>[2x]MSVLPGAAAIAGIGATEFSKNSGRSELQLACEAVLAAIADAGLEPSDVDGLVTFTADTSSEIHVARNTGIGELKFFSRVGYGGGAACGTVQQAAMAVATGIAEVVVCYRAFNERSGVRYGLGQAGRQMDQGADSAAYAWLLPFGLNTPAQWVAMFARRYMHEYGATSEDFGRVAVVDRKHAATNPKAWFYQRPITLEDHQNSRWIVEPLHLLDCCQESDGGQALVVVSTERARDLPHPPALIWGAAQGSGYDQHMMTSYYRSEITGIPEMGLVGQQLYAQSGLNPSDIGAAILYDHFTPLVLPQLEELGFCARGEAKDFIADGNLEIGGRLPCNTHGGQLGEAYIHGMNGIAEAVRLVRGTSVNQPGDVTNVLVTAGTGVPTSGLILGADRKLRSLEHHHHHH;>[2x]MRPAINRDNAFWFEAAKQRRLVIQRCA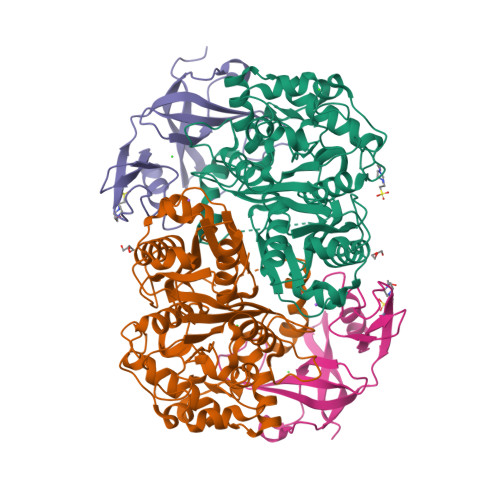ACKTLRHPPGPCCPHCGSFDWDTVEAAGTGQVYSYIVAHHPPHPAFEMPYVVALVELTEGTRLVTNLVGIAPDKIEIGMPVVLDWLEADPELTLPVFRPAVPQEES(2~{S},3~{S},4~{R},5~{S},6~{S})-2-[[(2~{S},4~{R},6~{R})-2-(hydroxymethyl)-6-oxidanyl-oxan-4-yl]methyl]-6-methyl-oxane-3,4,5-triol | C13 H24 O7 | 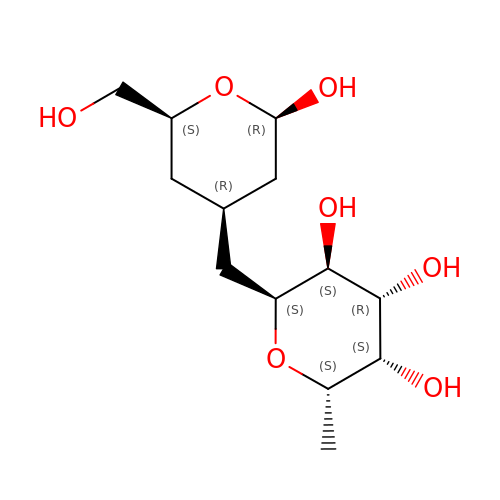ROOQANRWEBNDFF-VBFQFBHJSA-N> PIETVPVKLKPGMDGPKVKQWPLTEEKIKALVEICTEMEKEGKISKIGPENPYNTPVFAIKKKDSTKWRKLVDFRELNKRTQDFWEVQLGIPHPAGLKKKKSVTVLDVGDAYFSVPLDEDFRKYTAFTIPSINNETPGIRYQYNVLPQGWKGSPAIFQSSMTKILEPFRKQNPDIVIYQYMDDLYVGS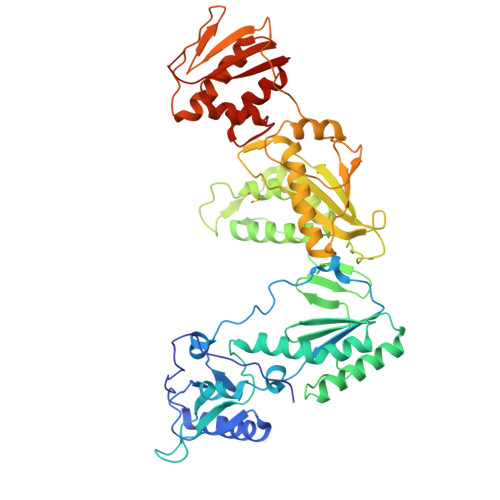DLEIGQHRTKIEELRQHLLRWGLTTPDKKHQKEPPFLWMGYELHPDKWTVQPIVLPEKDSWTVNDIQKLVGKLNWASQIYPGIKVRQLCKLLRGTKALTEVIPLTEEAELELAENREILKEPVHGVYYDPSKDLIAEIQKQGQGQWTYQIYQEPFKNLKTGKYARMRGAHTNDVKQLTEAVQKITTESIVIWGKTPKFKLPIQKETWETWWTEYWQATWIPEWEFVNTPPLVKLWYQLEKEPIVGAETFYVDGAANRETKLGKAGYVTNRGRQKVVTLTDTTNQKTELQAIYLALQDSGLEVNIVTDSQYALGIIQAQPDQSESELVNQIIEQLIKKEKVYLAWVPAHKGIGGN> MEIDYYDYEKLLEKAYQELPENVKHHKSRFEVP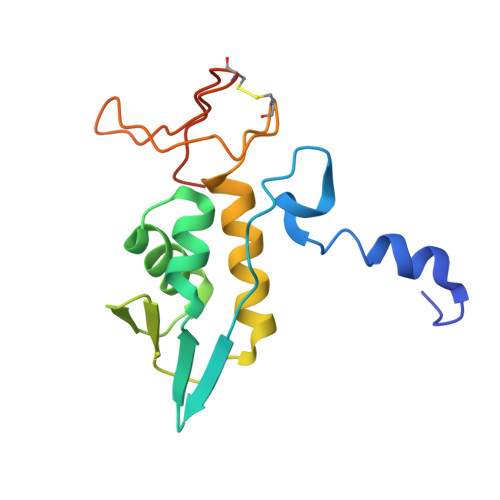GALVTIEGNKTIIENFKDIADALNRDPQHLLKFLLREIATAGTLEGRRVVLQGRFTPYLIANKLKKYIKEYVICPVCGSPDTKIIKRDRFHFLKCEACGAETPIQHLLEHHHHHH>MVF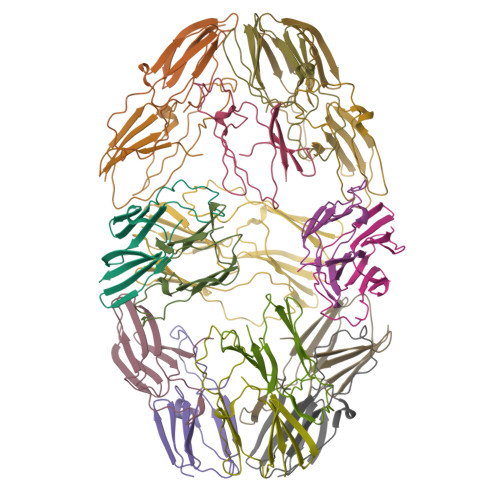ADSLFSDRFNRIDRLFSQLTGDTPVAATPAYDLQKRDANNYLLTVSVPGWKEEELEIETVGGNLNITGKHTEETVEDQTHWIYRGIRKADFQLSFSLPEHAKVNNAKLEQGLLLVEIYQEIPESEKPKKIAIES[6x]>SQNMDLTIGTHRESAFYELEFGPRTIMTLANFPDDVLPLLQMESLMTFEAMAYLRCDALVELGCYDGRALEIARLLNARYLGVDLDQRAIETLRTRIEREGMSDRADTVVDDILNHTRRGASVGSRALYLLPFNLLGNFREPKRLLDSLAERSVAAVVSVFGDSAEATRVRQSYYRRCGVQGLELHTRDDGTVFTGSDGFYSRSYSRACLHALLAECGLTVVRSASNLFAHCVTVLPEGADQGFGSSAA[2x]

AZE synthases catalyse the intramolecular 4-exo-tet cyclisation of S-adenosylmethionine (SAM), yielding a highly strained heterocycle. More recently, AZE synthases have been discovered in bacteria, namely AzeJ and VioH, which are involved in the biosynthesis of azetidomonamides and vioprolides, respectively. Interestingly, they show sequence similarity to the class I methyltransferases (MT1). Each subunit adopts a classic Rossmann fold, consisting of a 7-stranded β-sheet (β3↑, β2↑, β1↑, β4↑, β5↑, β10↓, β9↑) surrounded by helices α4-6, α8-9 and α11, a topology that is typical for MT1 enzymes.

Interestingly, the Fo-Fc electron density maps reveal that MTA and AZE are bound to the active site, suggesting that the substrate has been converted via an intramolecular nucleophilic nitrogen attack on the Cγ-carbon. Intriguingly, the structural superposition of AzeJ:SAH with AzeJ:MTA:AZE only shows marginal changes of the four-membered AZE-ring in the active site (rmsd = 0.3 Å, 221 Cα-atoms), except that the nitrogen and Cγ-atoms are moved by 1.5 Å towards each other. The amine group of AZE forms hydrogen bonds with the hydroxyl group of Tyr175 and the carbonyl oxygen of Phe134. Strong cation-π interactions with Phe134 indicate a protonated state of the nitrogen atom in the AZE product. Based on the atomic insights, we propose that during cyclisation the positive charge of the sulfonium group migrates to the C-N bond and accumulates on the AZE amine. This charge distribution is stabilised by cation-π interactions with Phe134, thereby facilitating the subsequent cleavage of the Cγ-S bond, which ultimately forms the neutral molecule MTA. Moreover, the AzeJ:MTA:AZE structure provides insights into how the α-amine of SAM, protonated under physiological conditions (SAM-NH3+), can be deprotonated. Similarly as seen in AzeJ:SAH, the carboxylate of AZE forms three hydrogen bonds with Asn139, Y176 and S203. The latter two residues further coordinate with Arg172, which is additionally H-bonded to Thr193 and a water molecule.> MEHVAFGSEDIENTLAKMDDGQLDGLAFGAIQLD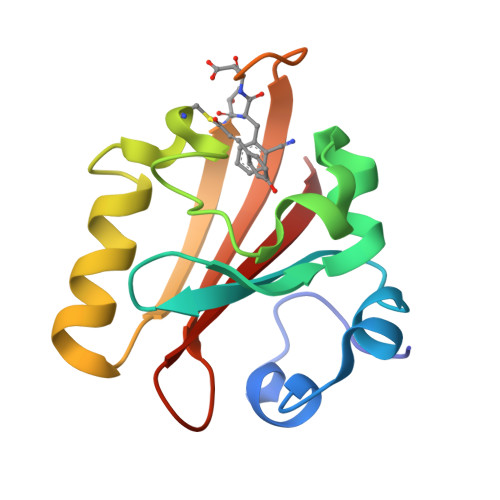GDGNILQYNAAEGDITGRDPKQVIGKNFFKDVAPCTDSPEFYGKFKEGVASGNLNTMFEYTXDYQETPTKVKVHMKKALSGDSYWVFVKRV> ADIIADADSPAKITIKANKLKDLKDYVDDLKTYNNTYSNVVTVAGEDRIETAIELSSKYYNSDDKNAITDDAVNNIVLVGSTSIVDGLVASPLASEKTAPLLLTSKDKLDSSVKSEIKRVMNLKSDTGINTSKKVYLAGGVNSISKDVENELKNMGLKVTRLSGEDRYETSLAIADEIGLDNDKAFVVGGTGLADAMSIAPVASQLKDGDATPIVVVDGKAKEISDDAKSFLGTSDVDIIGGKNSVSKEIEESIDSATGKTPDRISGDDRQATNAEVLKEDDYFKDG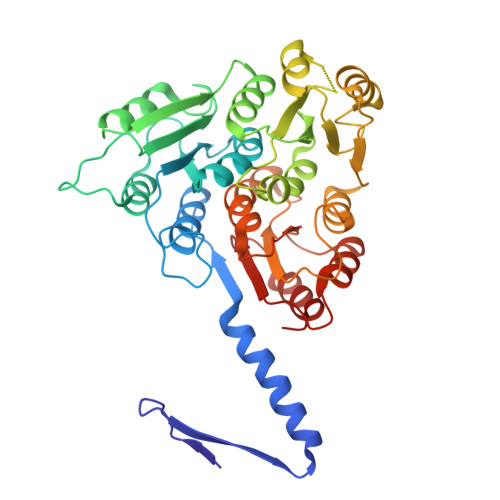EVVNYFVAKDGSTKEDQLVDALAAAPIAGRFKESPAPIILATDTLSSDQNVAVSKAVPKDGGTNLVQVGKGIASSVINKMKDLLDM>[2x]STRKAVIGYYF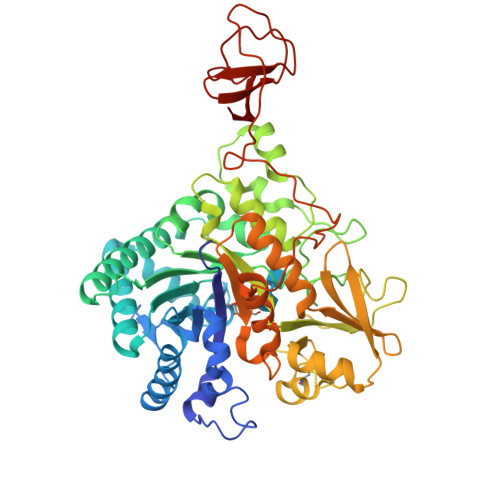IPTNQINNYTETDTSVVPFPVSNITPAKAKQLTHINFSFLDINSNLECAWDPATNDAKARDVVNRLTALKAHNPSLRIMFSIGGWYYSNDLGVSHANYVNAVKTPASRAKFAQSCVRIMKDYGFDGVDIDWEYPQAAEVDGFIAALQEIRTLLNQQTITDGRQALPYQLTIAGAGGAFFLSRYYSKLAQIVAPLDYINLMTYDLAGPWEKVTNHQAALFGDAAGPTFYNALREANLGWSWEELTRAFPSPFSLTVDAAVQQHLMMEGVPSAKIVMGVPFYGRAFKGVSGGNGGQYSSHSTPGEDPYPSTDYWLVGCEECVRDKDPRIASYRQLEQMLQGNYGYQRLWNDKTKTPYLYHAQNGLFVTYDDAESFKYKAKYIKQQQLGGVMFWHLGQDNRNGDLLAALDRYFNAADYDDSQLDMGTGLRYTGVGPGNLPIMTAPAYVPGTTYAQGALVSYQGYVWQTKWGYITSAPGSDSAWLKVGRVA> GAGCAGACAAG;> ACTTCACTCA;> CTAGT;> TCTGAGTGATGT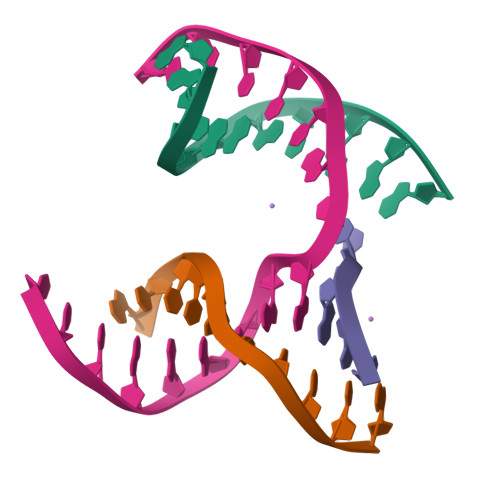CTGC> SWMEEVIKLCGRELVR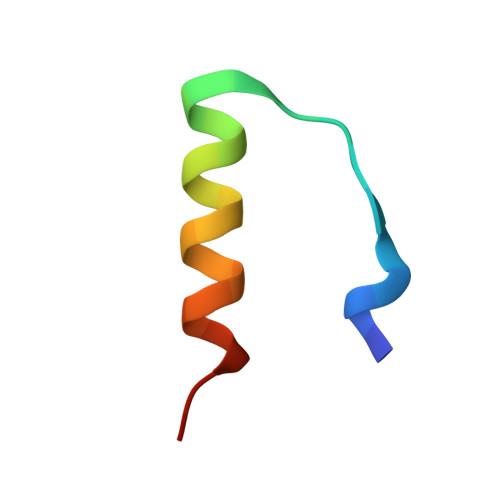AQIAICGMSTWS> MESKVVVPAQGKKITLQNGKLNVPENPIIPYIEGDGIGVDVTPAMLKVVDAAVEKAYKGERKISWMEIYTGEKSTQVYGQDVWLPAETLDLIREYRVAIKGPLTTPVGGGIRSLNVALRQELDLYICLRPVRYYQGTPSPVKHPELTDMVIFRENSEDIFAGIEWKADSADAEKVIKFLREEMGVKKIRFPEHCGIGIKPCSEEGTKRLVRAAIEYAIANDRDSVTLVHKGNI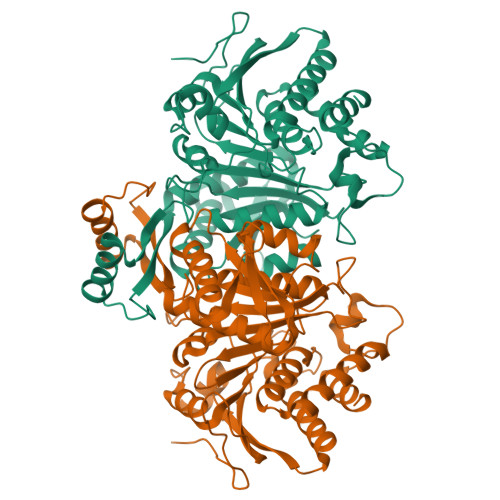MKFTEGAFKDWGYQLAREEFGGELIDGGPWLKVKNPNTGKEIVIKDVIADAFLQQILLRPAEYDVIACMNLNGDYISDALAAQVGGIGIAPGANIGDECALFEATHGTAPKYAGQDKVNPGSIILSAEMMLRHMGWTEAADLIVKGMEGAINAKTVTYDFERLMDGAKLLKCSEFGDAIIENM> MDLKGGESMVDWKLMQEIIEAPGVSGYEHLGIRDIVVDVLKEVADEVKVDKLGNVIAHFKGSSPRIMVAAHMDKIGVMVNHIDKDGYLHIVPIGGVLPETLVAQRIRFFTEKGERYGVVGVLPPHLRRGQEDKGSKIDWDQIVVDVGASSKEEAEEMGFRVGTVGEFAPNFTRLNEHRFATPYLDDRICLYAMIEAARQLGDHEADIYIVGSVQEEVGLRGARVASYAINPEVGIAMDVTFAKQPHDKGKIVPELGKGPVMDVGPNINPKLRAFADEVAKKYEIPLQVEPSPRPTGTDANVMQINKEGVATAVLSIPIRYMHSQ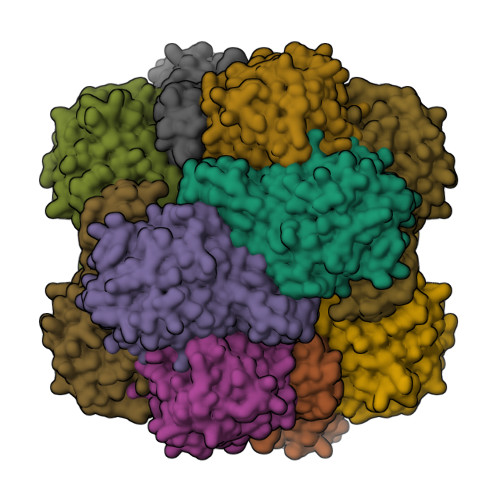VELADARDVDNTIKLAKALLEELKPMDFTP> SGRTWREADINYTSGFRNSDRILYSSDWLIYKTTDHYQTFT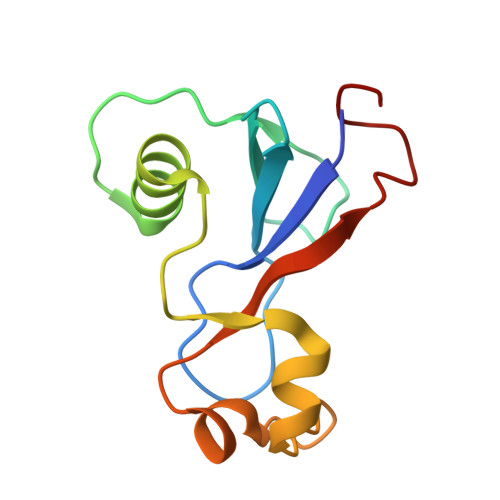KIRCAQVINTFDGVADYLQTYHKLPDNYITKSEAQALGWVASKGNLADVAPGKSIGGDIFSNREGKLPGK> 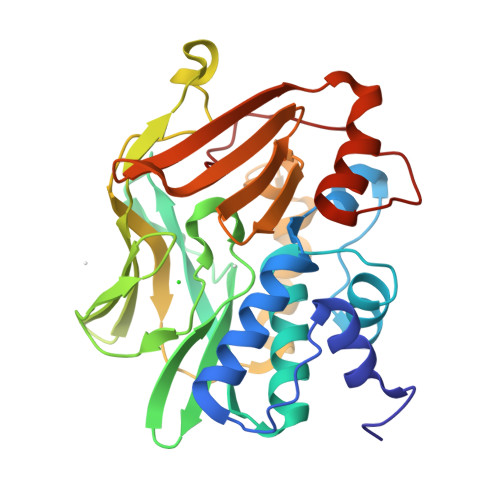GSGSGSDIEAYFERIGYKKSRNKLDLETLTDILQHQIRAVPFENLNIHCGDAMDLGLEAIFDQVVRRNRGGWXLQVNHLLYWALTTIGFETTMLGGYVYSTPAKKYSTGMIHLLLQVTIDGRNYIVDAGFGRSYQMWQPLELISGKDQPQVPCVFRLTEENGFWYLDQIRREQYIPNEEFLHSDLLEDSKYRKIYSFTLKPRTIEDFESMNTYLQTSPSSVFTSKSFCSLQTPDGVHCLVGFTLTHRRFNYKDNTDLIEFKTLSEEEIEKVLKNIFNISLQRKLVPKHGDRFFTI The hexanucleotide repeat expansion, GGGGCC (G4C2), within the first intron of the C9orf72 gene is known to be the most common genetic cause of both amyotrophic lateral sclerosis (ALS) and frontotemporal dementia (FTD). The G4C2 repeat expansions, either DNA or RNA, are able to form G-quadruplexes which induce toxicity leading to ALS/FTD. Here, we present the first crystal structures of an eight-layer parallel tetrameric G-quadruplex formed by two repeats of C9orf72 HRE DNA, d(G4C2)2, in Ba2+ and K+ solution, named as d(G4C2)2-Ba and d(G4C2)2-K respectively. Two d(G4C2)2 oligonucleotides form a parallel propeller-type dimeric G-quadruplex which stacks in a 5′-to-5′ arrangement making up a tetramer.

The crystal structure of d(G4C2)2-Ba in F222 space group was solved by a combination of molecular replacement and SAD method. The space group of d(G4C2)2-K is also F222 with similar cell dimensions, indicating they are isomorphous. Both d(G4C2)2-Ba (F222) and d(G4C2)2-K (F222) share similar structural features (with RMSD of core guanine residues of 0.243 Å) except the ions, thus we describe them here together. There are three chains, A-C in an asymmetric unit. Similar with the d(G4C2)2-Ba (C2221), two kinds of parallel-stranded tetrameric eight-layer G-quadruplexes were observed. The Form-1/1 stacking form was composed by chains B/C and their crystallographically symmetric chain Bsym/Csym. Notably, there are seven equal-spaced K+ ions lying along the axis within the central core of the tetrameric G-quadruplex including a well-defined central channel potassium ion located in the interface between the two dimeric blocks, while only four equal-spaced Ba2+ ions lying along the axis in the structure of d(G4C2)2-Ba (F222), which is exactly the same as the Ba2+ ions in the structure of d(G4C2)2-Ba (C2221). The crystal structures of d(G4C2)2-Ba in different space groups (i.e. C2221 and F222) have similar architecture, with the fact that the RMSD values of core guanine residues of Form-1/7 and Form-1/1 are 0.49 and 0.34 Å, respectively. The conformation of CC double-chain-reversal loops in d(G4C2)2-Ba2+ (F222) is also similar as d(G4C2)2-Ba2+ (C2221) and C·C+•C·C+ quadruple base pair and C•C·C+ triple base pair formed by the the 3′ end are also observed that stacks on the neighbouring dimeric blocks. Interestingly, a non-central channel Ba2+ is observed without close contact to DNA strand and water.

>[3x]GGGGCCGGGGCC PimE, the focus of our studies, is a polyprenyl-monophospho-β-d-mannose (PPM)-dependent mannosyltransferase that catalyzes the transfer of the fifth mannose from a PPM donor to the Ac1PIM4 acceptor substrate, leading to the formation of Ac1PIM5 via an α(1 → 2) glycosidic bond. PimE contains twelve TM helices with both the N- and C-termini located on the cytoplasmic side of the membrane. PimE belongs to the GT-CA subclass of glycosyltransferases, characterized by a conserved core module of seven TM helices. PimE, like many other structurally characterized GT-C enzymes, is an inverting glycosyltransferase, which is thought to operate through a single-step nucleophilic substitution mechanism facilitated by an enzymatic general base catalyst and can occur in either a metal-dependent or independent way.

In this study, we used single-particle cryo-electron microscopy (cryo-EM) to determine high-resolution structures of PimE in the apo form and in a complex bound with its mannosylated product Ac1PIM5 and by-product PP at 3.0 and 3.5 Å resolution, respectively. The phosphate group of PP is located along the cationic half of the cavity. At the same time, the mannose head of Ac1PIM5 is positioned along the anionic half. Only the first three prenyl units of the polyprenyl chain of PP could be resolved, with the chain pointing towards the hydrophobic groove between TM helices 6 and 9. Our structure reveals a network of interactions between PimE and its ligands. At the center of the binding pocket, D58, located at the tip of JM1, forms a hydrogen bond with the C2 hydroxyl group of the fifth mannose of Ac1PIM5. Y62 forms a hydrogen bond with D58, potentially stabilizing its orientation within the active site. The phosphate group of PP is coordinated by three conserved residues, H322, W319, and K195. K195 forms a salt bridge with the phosphate, while H322 forms a hydrogen bond with one of the phosphate oxygens.

> MATEKTEPTRANVEPPMPTRGASAWRRVRAWGPWLLGLSVAVRLAWAYLTPHGADLVDLHVYVSGPATLGHGNLYEFTYPDKTPDFPLPFTYPPFAAVVFWPLHLIPFTLLGLCWILGTIAALYAVVRLSQRLLGFDDARAAAVWTAVTMWTEPVRSTLDYGQINVLLMLLILLAVASSRWWISGTLIGLAGGVKLTPLVSGLYFLGARRWTTAIWAGVVFLLTVVVGIAVVGEQGRYYFTDLLGKPDRIGPIATVFNQSWRGGISRILGHDAGSGVLVLFAYAVTAILAFLAWRAVNDRLGQICVVEMFGLLISPISWTHHWVWMVPFMVWLLHGPWRDKVGAKVFGCGWLVLLLIGVPWLLSFAQPDIWRIDRPWPLAWAGLVDIVAAIATLTWMAVVGRRSGHLGRLPWRHV>[2x]MSMLGERRRGLTDPEMAAVILKALPEAPLDGNNKMGYFVTPRWKRLTEYEALTVYAQPNADWIAGGLDWGDW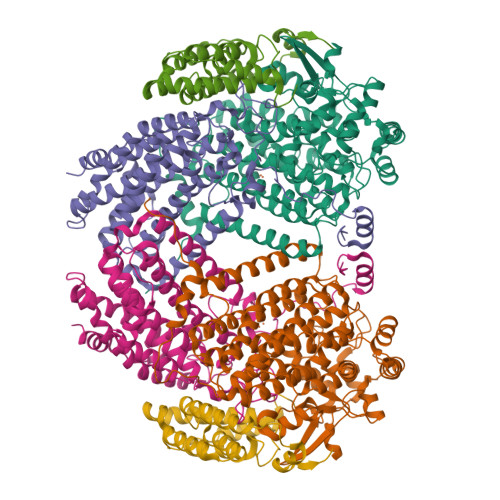TQKFHGGRPSWGNETTELRTVDWFKHRDPLRRWHAPYVKDKAEEWRYTDRFLQGYSADGQIRAMNPTWRDEFINRYWGAFLFNEYGLFNAHSQGAREALSDVTRVSLAFWGFDKIDIAQMIQLERGFLAKIVPGFDESTAVPKAEWTNGEVYKSARLAVEGLWQEVFDWNESAFSVHAVYDALFGQFVRREFFQRLAPRFGDNLTPFFINQAQTYFQIAKQGVQDLYYNCLGDDPEFSDYNRTVMRNWTGKWLEPTIAALRDFMGLFAKLPAGTTDKEEITASLYRVVDDWIEDYASRIDFKADRDQIVKAVLAGLK;>[2x]MALSTATKAATDALAANRAPTSVNAQEVHRWLQSFNWDFKNNRTKYATKYKMANETKEQFKLIAKEYARMEAVKDERQFGSLQDALTRLNAGVRVHPKWNETMKVVSNFLEVGEYNAIAATGMLWDSAQAAEQKNGYLAQVLDEIRHTHQCAYVNYYFAKNGQDPAGHNDARRTRTIGPLWKGMKRVFSDGFISGDAVECSLNLQLVGEACFTNPLIVAVTEWAAANGDEITPTVFLSIETDELRHMANGYQTVVSIANDPASAKYLNTDLNNAFWTQQKYFTPVLGMLFEYGSKFKVEPWVKTWNRWVYEDWGGIWIGRLGKYGVESPRSLKDAKQDAYWAHHDLYLLAYALWPTGFFRLALPDQEEMEWFEANYPGWYDHYGKIYEEWRARGCEDPSSGFIPLMWFIENNHPIYIDRVSQVPFCPSLAKGASTLRVHEYNGQMHTFSDQWGERMWLAEPERYECQNIFEQYEGRELSEVIAELHGLRSDGKTLIAQPHVRGDKLWTLDDIKRLNCVFKNPVKAFN;>[2x]MAKLGIHSNDTRDAWVNKIAQLNTLEKAAEMLKQFRMDHTTPFRNSYELDNDYLWIEAKLEEKVAVLKARAFNEVDFRHKTAFGEDAKSVLDGTVAKMNAAKDKWEAEKIHIGFRQAYKPPIMPVNYFLDGERQLGTRLMELRNLNYYDTPLEELRKQRGVRVVHLQSPH>[2x]SMPACDEFDQLIKNMAQGRHVEVFELLKPPSGGLGFSVVGLRSENRGELGIFVQEIQ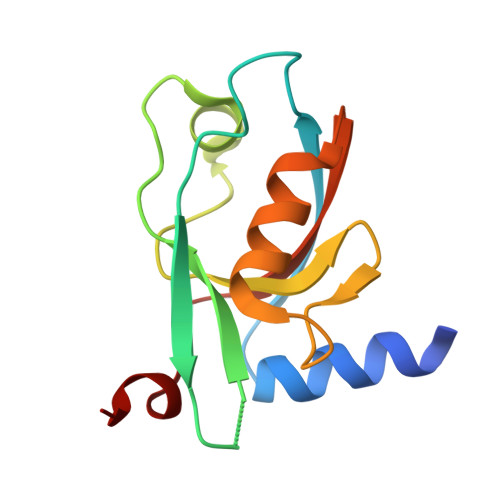EGSVAHRDGRLKETDQILAINGQALDQTITHQQAISILQKAKDTVQLVIARGSLPQYYKV>SNAMRQRTIVCPLI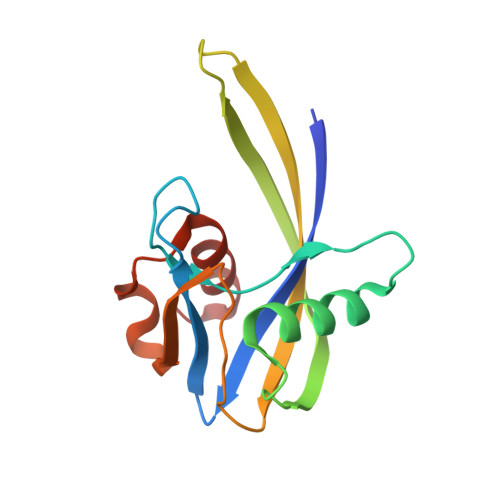QNDGCYLLCKMADNRGVFPGQWALSGGGVEPGERIEEALRREIREELGEQLILSDITPWTFRDDIRIKTYADGRQEEIYMIYLIFDCVSANRDICINDEFQDYAWVAPAALALYDLNVATRHTLALKGLL[2x]>HEHNTIPKGASIEVKVQQLDPVNGNKDVGTVTITESNYGLVFTPDLQGLSEGLHGFHIHENPSCEPKEQEGQLTAGLGAGGHWDPKGAKQHGYPWQDDAHLGDLPALTVLHDGTATNPVLAPRLKHLDDVRGHSIMIHTGGDNHSDHPAPLG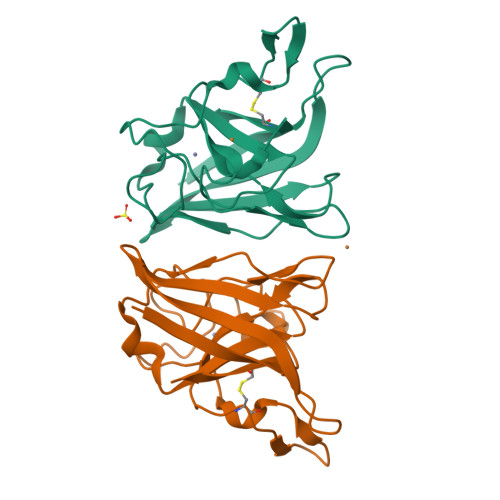GGGPRMACGVIK[3x]>[2x]MTINYQFGDVDAHGAMIRAQAGLLEAEHQAIVRDVLAAGDFWGGAGSVACQEFITQLGRNFQVIYEQANAHGQKVQ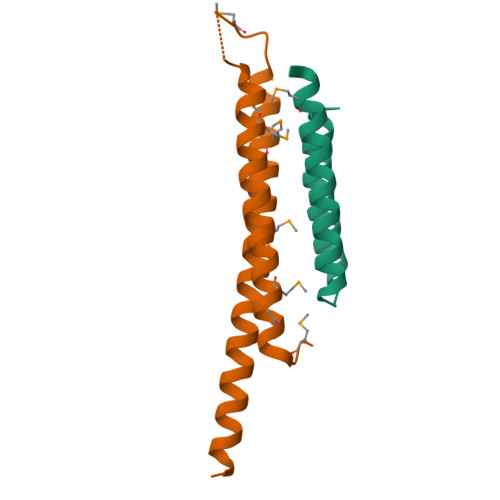AAGNNMAQTDSAVGSSWATHHHHHH;>[2x]SMATRFMTDPHAMRDMAGRFEVHAQTVEDEARRMWASAQNISGAGWSGMAEATSLDTMAQMNQAFRNIVNMLHGVRDGLVRDANNYEQQEQASQQILSS PUF (for Pumilio and FBF) RNA-binding proteins regulate gene expression post-transcriptionally throughout Eukarya. The signature biochemical activity of all PUF proteins is sequence-specific binding to defined RNA regulatory elements. They do so via an RNA-binding domain (RBD) spanning eight α-helical repeats, called PUF or Pumilio repeats. The FBF RBD can recognize either of two core elements: a longer ‘canonical’ 9-nt FBE with a consensus sequence of 5′-UGURnnAUn-3′ (R=purine)23–26 or a shorter compact 8-nt FBE (cFBE) with the consensus 5′-UGUGAA(A/U)n-3′21,27.

A candidate emerged just three nucleotides downstream of FBEa. Its sequence (5′-CAUGUUGCCAUU-3′) contained key FBE features (boldface): a 5′ UGU, 3′ AU, and an upstream C, and these features are conserved among Caenorhabditids. The candidate sequence deviated from a canonical FBE: a uridine followed the UGU, rather than typical purine, and a second uridine replaced the typical final adenosine. We first determined a 2.2 Å resolution crystal structure of the FBF-2 RBD in complex with an 11-nt RNA carrying FBEa*. Indeed, FBF-2 bound to FBEa* by recognizing the 5′ and 3′ nucleotides common to FBEa and FBEa*: FBF-2 interacts with 5′-CAUGU and CCAU-3′ in both FBEa and FBEa*. The FBF-2 RBD structure changes little (RMSD = 0.37 Å over 2, 744 atoms). The RNA sequences align in the 5′ and 3′ regions, and the side chains that contact the RNA bases in each structure are equivalent and positioned similarly. No electron density was seen for the atypical U4 base of FBEa* (cyan arrow), so U4 is likely flipped away from the RNA-binding surface, as seen with other PUF binding elements with flipped bases. Following the flipped U4 nucleotide, PUF repeat 5 (R5) interacted with G5 of FBEa* in a manner similar to its interaction with G4 of FBEa. We next measured FBF-2 binding affinities to a 14-nt RNA carrying FBEa* using an electrophoretic mobility shift assay (EMSA). Despite equivalent contacts with the two RNAs, FBF-2 RBD bound to FBEa* RNA with a KD = 427 nM (Fig. 2f, line 1), ~6-fold weaker than its previously reported binding to FBEa RNA (KD = 70 nM).

> GSNNVLPTWSLDSNGEMRSRLSLSEVLDSGDLMKFAVDKTGCQFLEKAVKGSLTSYQKFQLFEQVIGRKDDFLKLSTNIFGNYLVQSVIGISLATNDDGYTKRQEKLKNFISSQMTDMCLDKFACRVIQSSLQNMDLSLACKLVQALPRDARLIAICVDQNANHVIQKVVAVIPLKNWEFIVDFVATPEHLRQICSDKYGCRVVQTIIEKLTADSMNVDLTSAAQNLRERALQRLMTSVTNRCQELATNEYANYIIQHIVSNDDLAVYRECIIEKCLMRNLLSLSQEKFASHVVEKAFLHAPLELLAEMMDEIFDGYIPHPDTGKDALDIMMFHQFGNYVVQCMLTICCDAVSGRRQTKEGGYDHAISFQDWLKKLHSRVTKERHRLSRFSSGKKMIETLANLRSTHPIYELQ> MNLTDSLQNVLSGVGTLNRYRLDIPSCPSSLDVEDFSGTEGISKIYRYDIIFTSTDRYPDAAWFLRKSATLIMGTGLLESLTEQKKVHGVITDFRRISGSEDQAQYRITLKPFISLLDKQFRTHRFFVNKSVPEVVEQILTEHGLKGWEYEFSLKRTYPKREQINQYQESDLRFIQRLLAEVGIFYFFTLHPDAQTEVIHFGDVQAALIFDKTLPVNSPSGMSDSGTDSVWALNVEHRVVESRVITNDYNHREAQNILMSVPADMTRGEGYDTSYGEVYHYRPRHTERGDKIDPAPETANFWARLDHERFLAEQTRITGKSTDASLLPAQVLTITDSTPPVLPAPLQEPVLLTQLLFTGSRKSALQVMLSAVPYSEIVCWRPPLLTRPKITGTMTARVTSAKEGDIYAWQDASGMYRVKFDADRDDKNPGQESMPVRLAKPYSGDAYGFHFPLIQGTEVAIAFEEGDPDRPYIAHALHDSRHVDHVTDKNGTRNVIRTPANNKLRMEDKRGEEHIKLSTEYGGKTQLNLGHNVDASRELRGEGAELRTDDWISIRGGKGIFISADMQPQAQGKMLDMDEAIRQLEQALSLARSMAKAATAANATQGDISCQQRLNASLTDLTAPGMLLHAPDGIGMVSARALRIASGSESVGIMSGDNTDITAGQSFTVVAEGAVSLLSRNQGMQLLAAKGRVNIQAQSDDLSMSSQQNLDIQSSEGKVTVSANQELILACGGAYIKLSGGNIELGCPGQILLKSTNMQKMGPTSLDIASVEMPRGFGGGFILTDEAGVPQPSTPYRLTTAEGDILQGITDENGKTAPVNTSIPSVVKVEFGKVKIHGETE;> MTKYQGYDVTDATHKTSIHNDWKVVVAKKKPARGVTLTIGIFFDGTGNNRENTASRLMKFNECSA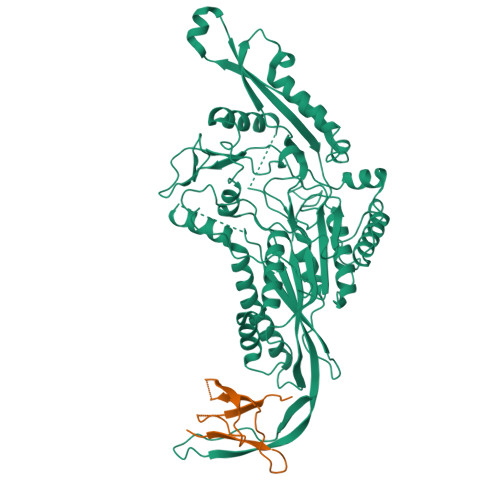ARQGVNQKDAQSCEDFLKEINKNSISNGSYRGYYSNIHWLNILYHPDQVLKKDQTSAQIKTYISGIGTAAGEADSVIGMGLGTSILDIFEGVVTKTDEAMERITQALSEFMGFNLSPDFCIAKIQFDVFGFSRGAAAARHFANRVMEQDPAIARAIAKGLRGDFYDGKPSGEVRFLGLFDTVAAIGGISNFFDINGRSNPGVKLELRPSVAKKVFQITAMNEYRYNFSLNSIKGMWPELALPGAHSDIGGGYNPVGSPLQENESLFLSCPEFEIVSDDTREMDTRVYRKAEQVRKMLMTLPALKHILPHGKLTTKIRSIGVNNSNQRRAGVIQKQVGAAVFFERMAVPNDWANVCLRVMLDAAQEAGVLFEPIRQTNTELQLPSELIFLADKAIAQGKAVRLGQEPQAFTEEELYIIGKYTHCSANWNIESDGNLWVDPTTGEIFIHRFGPKGNKAFVFPNKPNDRWIRSVWYMDDQQRLNDNAVKNTKVMMSGV NF-κB is a family of evolutionarily conserved transcription factors that provide stimulus-dependent temporal control over target gene expression. Despite its original characterization as a repressor of target gene transcription, the NF-κB p50 homodimer was subsequently shown to be an active transcription factor through its association with other nuclear factors, such as the IκBζ co-activator protein. By virtue of its low affinity for cytoplasmic IκB protein inhibitors, p50 accumulates in the nucleus of resting cells, where it is a binding target for the transcriptional co-activator IκBζ. The resulting crystallographic model reveals the well-characterized DNA-binding NF-κB RHR (also commonly referred to as the “RHD”) composed of an amino-terminal domain (murine p50 residues 39–239) and a short interdomain linker (residues 240–247) followed by the dimerization domain (residues 248–350).

To address these questions, we engineered a “Test” DNA containing the core κB-like sequence 5′-GGGGAATTCCCC-3′. We embedded this core sequence within ends of different sequence and length so as to impose asymmetry in crystal packing and unambiguous identification of DNA orientation during model-building and crystallographic refinement and determined the X-ray crystal structure of the resulting 16-mer DNA in complex with p50 at 3.0 Å resolution. The resulting crystallographic model clearly reveals that p50 binds the Test κB-like DNA with 11-bp spacing. Moreover, since the Test DNA does not contain a central A:A mismatch, the binding is inherently asymmetric. Base-specific contacts between p50:Test and p50:IL-6 are largely conserved. One notable difference is that, in the p50:Test complex, Lys241 from subunit A binds to the available fourth G base, as expected. Lys241 from subunit B contacts the T base of a T:A bp, just as it does in the p50:IL-6 complex. This is significant because, if the p50 homodimer bound DNA with 12-bp spacing, then it could accommodate both triplet G binding by the loop L1 residues and a second favored Lys241:G interaction by subunit B. Rather, p50 binds to the Test κB DNA with 11-bp spacing. Therefore, the p50:Test complex X-ray crystal structure strongly suggests that 11-bp spacing to κB DNA is the preferred binding mode by the NF-κB p50 homodimer. Furthermore, it illustrates how the preferred binding of a two-fold symmetric p50 homodimer dimer to 11-bp within a two-fold symmetric κB DNA necessarily introduces asymmetry into an otherwise symmetrical complex.

>[2x]GPYLQILEQPKQRGFRFRYVCEGPSHGGLPGASSEKNKKSYPQVKICNYVGPAKVIVQLVTNGKNIHLHAHSLVGKHCEDGVCTVTAGPKDMVVGFANLGILHVTKKKVFETLEARMTEACIRGYNPGLLVHSDLAYLQAEGGGDRQLTDREKEIIRQAAVQQTKEMDLSVVRLMFTAFLPDSTGSFTRRLEPVVSDAIYDSKAPNASNLKIVRMDRTAGCVTGGEEIYLLCDKVQKDDIQIRFYEEEENGGVWEGFGDFSPTDVHRQFAIVFKTPKYKDVNITKPASVFVQLRRKSDLETSEPKPFLYYPE Here, we study fold transition between distinct β-barrels by protein engineering and structural biology technique. Here, we discover that the previously reconstructed ancient DPBB sequence could also adopt a β-barrel fold named Double-Zeta β-barrel (DZBB), as a metamorphic protein. The DZBB fold is not found in any modern protein, although its structure shares similarities with RIFT and OB. Furthermore, the reconstructed OB fold could also be converted to the four-stranded SH3 fold by a simple circular permutation. Thus, these ancient β-barrel folds (DPBB, RIFT, OB, and SH3) could be readily interconverted by a few feasible mutations through the missing-link fold, DZBB, indicating their significantly close evolutionary relationships.

The most simplified DPBB protein we designed previously, design-1 (mk2h_ΔMILPYS), did not fold in the typical buffer conditions (50 mM phosphate, 150 mM NaCl), but crystallized under two different conditions, containing malonate or malic acid ions, and adopted the DPBB fold in the crystals. Here, we report its third type of crystal, formed under different conditions (100 mM Tris, pH8.5, 20% PEG-400, 200 mM lithium sulfate). Interestingly, we could not solve its structure by molecular replacement using the DPBB fold as a model, implying that design-1 had adopted a different conformation in the third type of crystal. By molecular replacement with the predicted design-2 model (RIFT fold) and subsequent manual remodeling, the crystal structures of design-1 (third type of crystal) and design-2 were determined. Surprisingly, they both adopted into a unique β-barrel fold that topologically differs from DPBB and RIFT. Compared to the homo-dimeric DPBB fold, the directions of the β2- and β2’-strands were inverted, resulting in all anti-parallel strand patterns like those in RIFT. However, the 1st loop connecting β1– β2 was rolled up, unlike the simple β-turn in RIFT. As this loop configuration resembles the letter “Zeta” in the topological scheme, we named this β-barrel fold the Double-Zeta β-barrel (DZBB). Therefore, design-1 can fold into two different structures with an identical sequence. Design-1 exhibited the metamorphic property, adapting two different folds, DPBB and DZBB.

> GPMPGKKVVARVAEARAEDVGKRVVRVDKAERAKVGVKVGDVVEVKKV>DVSGTVCLSALPPEATDTLNLIASDGPFPYSQDGVVFQNRESVLPTQSYGYYHEYTVITPGARTRGT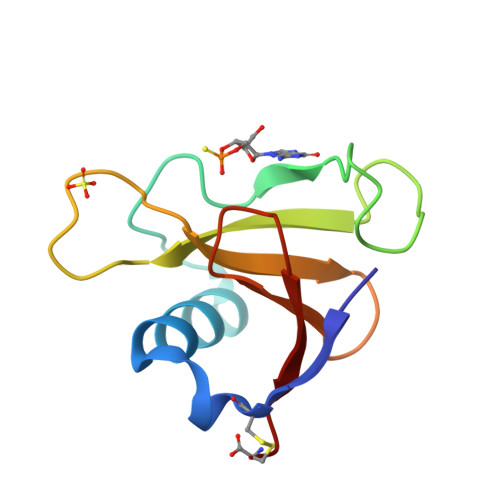RRIICGEATQEDYYTGDHYATFSLIDQTC[2x]> CGGPFELWEPNTTFSSTNFPNSYPNLAFCVWILNAQKGKNIQLHFQEFDLENINDVVEIRDGEEADSLLLAVYTGPGPVKDVFSTTNRMTVLLITNDVLARGGFKANFTTGYHLGIPEPCKADHFQCKNGECVPLVNLCDGHLHCEDGSDEADCVRFFNGTTNNNGLVRFRI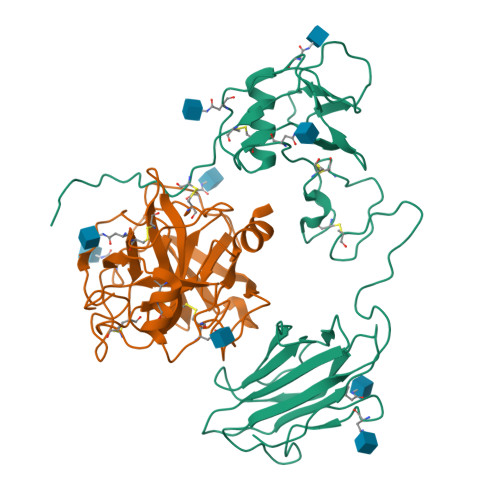QSIWHTACAENWTTQISNDVCQLLGLGSGNSSKPIFPTDGGPFVKLNTAPDGHLILTPSQQCLQDSLIRLQCNHKSCGKKLAAQDITPK;> IVGGSNAKEGAWPWVVGLYYGGRLLCGASLVSSDWLVSAAHCVYGRNLEPSKWTAILGLHMKSNLTSPQTVPRLIDEIVINPHYNRRRKDNDIAMMHLEFKVNYTDYIQPICLPEENQVFPPGRNCSIAGWGTVVYQGTTANILQEADVPLLSNERCQQQMPEYNITENMICAGYEEGGIDSCQGDSGGPLMCQENNRWFLAGVTSFGYKCALPNRPGVYARVSRFTEWIQSFLH>GMSHIQRETSCSRPRLNSNLDADLYGYRWARDNVGQSGATIYRLYGKPNAPELFLKHGKGSVANDVTDEMVRL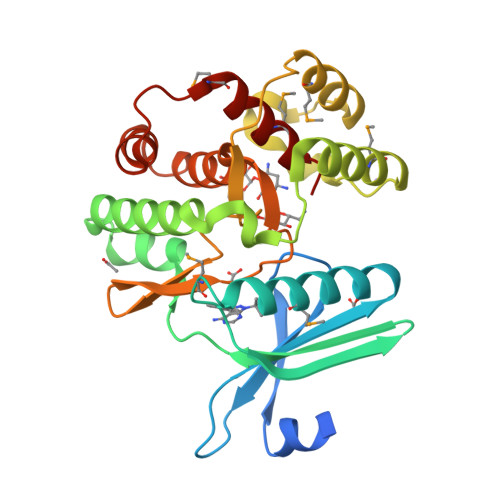NWLTAFMPLPTIKHFIRTPDDAWLLTTAIPGKTAFQVLEEYPDSGENIVDALAVFLRRLHSIPVCNCPFNSDRVFRLAQAQSRMNNGLVDASDFDDERNGWPVEQVWKEMHKLLPFSPDSVVTHGDFSLDNLIFDEGKLIGCIDVGRVGIADRYQDLAILWNCLGEFSPSLQKRLFQKYGIDNPDMNKLQFHLMLDEFF[12x]> MNGQHPRSVVTAPDATTGTTSYDVVVVGAGIAGLYAIHRFRSQGLTVRAFEAASGVGGVWYWNRYPGARCDVESIDYSYSFSPELEQEWNWSEKYATQPEILAYLEHVADRFDLRRDIRFDTRVTSAVLDEEGLRWTVRTDRGDEVSARFLVVAAGPLSNANTPAFDGLDRFTGDIVHTARWPHDGVDFTGKRVGVIGTGSSGIQSIPIIAEQAEQLFVFQRSANYSIPAGNVPLDDATRAEQKANYAERRRLSRESGGGSPHRPHPKSALEVSEEERRAVYEERWKLGGVLFSAAFPDQLTDPAANDTARAFWEEKIRAVVDDPAVAELLTPKDHAIGAKRIVTDSGYYETYNRDNVELVDLRSTPIVGMDETGIVTTGAHYDLDMIVLATG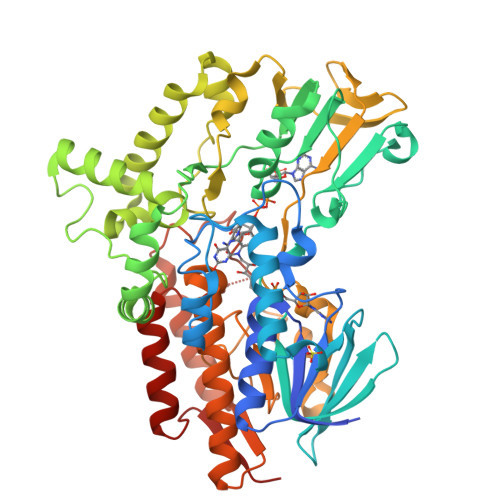FDAMTGSLDKLEIVGRGGRTLKETWAAGPRTYLGLGIDGFPNFFNLTGPGSPSVLANMVLHSELHVDWVADAIAYLDARGAAGIEGTPEAVADWVEECRNRAEASLLNSANSWYLGANIPGRPRVFMPFLGGFGVYREIITEVAESGYKGFAILEG> GLGDLIEGVVEGVTRNALTPLTPANNL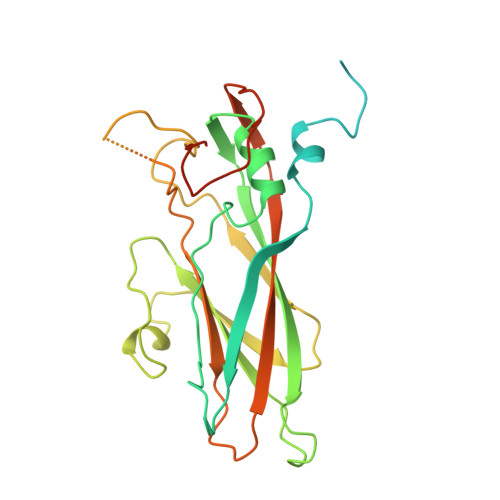PDTQSSGPAHSKETPALTAVETGATNPLVPSDTVQTRHVIQKRTRSESTVESFFARGACVAIIEVDNDAPTKRASKLFSVWKITYKDTVQLRRKLEFFTYSRFDMEFTFVVTSNYTDANNGHALNQVYQIMYIPPGAPIPGKWNDYTWQTSSNPSVFYTYGAPPARISVPYVGIANAYSHFYDGFAKVPLAGQASTEGDSLYGAASLNDFGSLAVRVVNDHNPTKLTSKIRVYMKPKHVRVWCPRPPRAVPYYGPGVDYKDGLAPLPEKGLTTY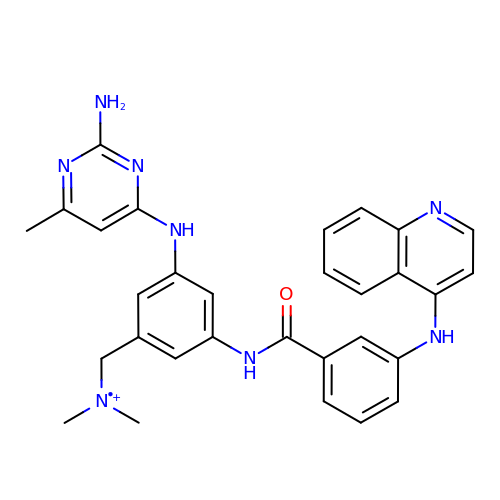N-{3-[(2-amino-6-methylpyrimidin-4-yl)amino]-5-[(dimethylamino)methyl]phenyl}-3-[(quinolin-4-yl)amino]benzamide | C30 H30 N8 O | FJKSIMNYGCBSRZ-UHFFFAOYSA-O> MDNQCTVQVRLELGHRAQLRKKPTTEGFTHDWMVFVRGPEQCDIQHFVEKVVFWLHDSFPKPRRVCKEPPYKVEESGYAGFIMPIEVHFKNKEEPRKVCFTYDLFLNLEGNPPVNHLRCEKLTFNNPTTEFRYKLLRAGGVM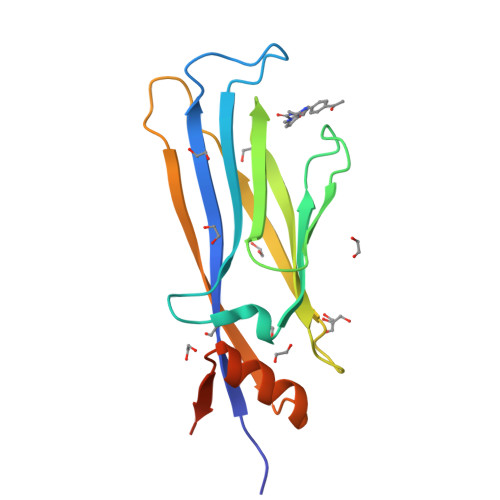VMPEGAHHHHHH>[2x]MTTGLSTAGAQDIGRSSVRPYLEECTRRF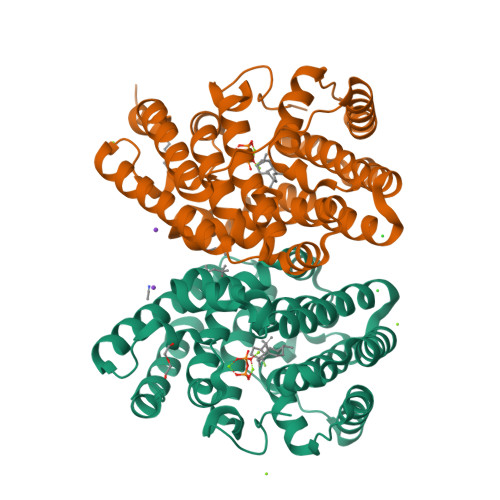QEMFDRHVVTRPTKVELTDAELREVIDDCNAAVAPLGKTVSDERWISYVGVVLWSQSPRHIKDMEAFKAVCVLNCVTFVWDDMDPALHDFGLFLPQLRKICEKYYGPEDAEVAYEAARAFVTSDHMFRDSPIKAALCTTSPEQYFRFRVTDIGVDFWMKMSYPIYRHPEFTEHAKTSLAARMTTRGLTIVNDFYSYDREVSLGQITNCFRLCDVSDETAFKEFFQARLDDMIEDIECIKAFDQLTQDVFLDLIYGNFVWTTSNKRYKTAVNDVNSRIQAAALEHHHHHH>MDEYVQELKGLIRKHIPERCEFGHQKVTFLSQVHPSPLLTEGFKLLSSLVELESCEAHACQANTDQRFVDVILSDNGILCPTLPKVIPDGFKLTGKTLILLETFVRVNPDEFEKKWKADMSKLLNLKHDLQKSGVTLVPIVDGRSNYNNRFVADWVIERIRWLLIEILKASKSMLEIDIEDQEYQRLIHSLSNVKNQSLGLENLEHLKRNSLDYDERLNESLFIGLKGDIRESTVREELIKLKLWFKDEVFSKGLGKFKLTDRRELLESLSSLGAHLDSDVSSCPFCNNKLMEIVYNVTFSCVERTDGVATVDQQFSTTHSNIEKHYLSVLSLCNKIKGLKVFNTRRNTLLFLDLIMVNLMVDISDSCQDAIESLRKSGLIVGQMVMLVNDRVLDILEAVKLIRKKIGTNPNWVKNCSKILERSHPEIWHHLSTLIKQPDFNSLISIAQHLVSDRPIMRYSVERGSDKICRHKLFQEMSSFEQMRLFKTLSSISLSLINSMKTSFSSRLLVNEREFSKYFGNVRLRECYAQRFYLAESLVGFLFYQKTGERSRCYSVYLSDNGVMSEQGSFYCDPKRFFLPVFSDEVLAGMCEEMTSWLDFDTGLMNDTGPILRLLVLAILCSPSKRNQTFLQGLRYFLMAFANQIHHIDLTSKLVVECKSSSEVVVQRLAVGLFIRLLSGESDASLFFSRRFKYLLNVSYLCHLITKETPDRLTDQIKCFEKFIEPKVKFGCAVVNPSLNGKLTVDQEDIMINGLKKFFSKSLRDTEDVQTPGVCKELLNYCVSLFNRGKLKVSGELKNNPFRPNITSTALDLSSNKSVVIPKLDELGNILSTYDKEKLVSACVSSMAERFKTKGRYNLDPDSTDYLILKNLTGLVSAGPKAKSTQEELSLMYEALTEEQVESFNEIKHDVQVALAKMADNSVNTRTKNLGRADNSVKNGNNPLDNLWSPFGVMKEIRAEVSLHEVKDFDPDVLPPEVYKELCDAVYKSSEKCNFFLEGVLDVCPLGLLLKNLTTSSYVDEEYFMCFKYLLIQGHFDQKLGSYEHKSRSRLGFTDETLRLKDEVRLSIRESNSEAIADKLDKSYFTNAALRNLCFYSEDSPT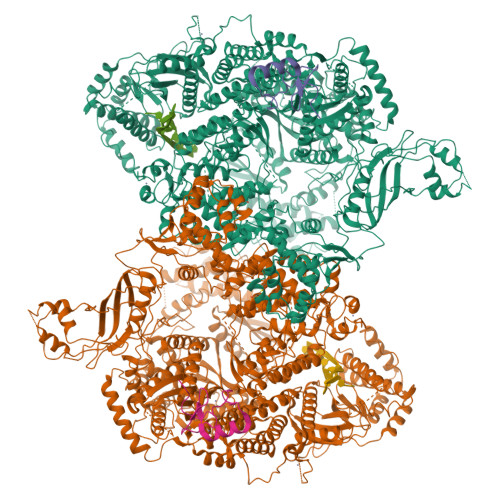EFTSISSNSGNLKFGLSYKEQVGSNRELYVGDLNTKLMTRLVEDFSEAVGNSMKYTCLNSEKEFERAICDMKMAVNNGDLSCSYDHSKWGPTMSPALFLALLQMLELRTPVDRSKIDLDSVKSILKWHLHKVVEVPINVAEAYCIGKLKRSLGLMGCGSTSLSEEFFHQTMQLNGQIPSHIMSVLDMGQGILHNTSDLYGLITEQFLCYALDLLYDVIPVSYTSSDDQITLIKTPSLDIEGGSDAAEWLEMICFHEFLSSKLNKFVSPKSVIGTFVAEFKSRFFVMGEETPLLTKFVAAALHNVKCKTPTQLSETIDTICDQCIANGVSTKIVTRISKRVNQLIRYSGYGETPFGAIEDQDVKDWVDGSRGYRLQRKIEAIFHDDKETSFIRNCARKVFNDIKRGRIFEENLINLIGRGGDEALTGFLQYAGCSEQEVNRVLNYRWVNLSSFGDLRLVLRTKLMTSRRVLEREEVPTLIKTLQSKLSRNFTKGVKKILAESINKSAFQSSVASGFIGFCKSMGSKCVRDGKGGFLYIKEVYSGVSACTCEICALKPKIIYCNNSLNKVSQFSKPILWDYFSLVLTNACELGEWVFSTVKEPQKPLVLNNQNFFWAVKPKVVRQIEDQLGMNHVLQSIRRNYPVLFDEHLTPFMNDLQVSRTMDSGRLKFLDVCIALDMMNENLGIISHLLKTRDNSVYIVKQSDCALAHIRQSSYTDWELGLSPQQICTNFKTQLVLSSMVNPLVLSTSCLKSFFWFNEVLELEDDSQIELAELTDFALMVKNQNVSRAMFVEDIAMGYVVSNFEGVRISLSNVMVDGVQLPPQEKAPDIGELFGLKAENVIVGLVVQIDHVRMSTKFKLKRKMVYSFSLECIMDVGEIQNKEVILKVVAVDQSVSGSGGNHMLLDGVSVVASLPLFTGQASFDLAAMLIESNLAGSNDNFLMRNVTLDLGGFSPELSDKYSYRLSGPENQEDPLVLKDGAFYVGGERLSTYKVEFTGDLVVKALGALEDDESVVSMLHQLWPYLKATSQVILFQQEDFTIVHDLYKKQLTKSIESFGEWIEFTNFKVAYSKSLKELVISDTQGSFRLKGVMCRPLASTPQVEDIE[2x];>MGNCNKPPKRPPNTQTSSNQPSAEFRRTAPPSLYGRYNCKCCWFADTNLITCNDHYLCLRCHQTMLRNSELCHICWKPLPTSITVPVEPSAPPP[2x]5-(2,2,2-Trifluoro-ethoxy)-pyridine-2-carboxylic acid [3-((S)-2-amino-1,4-dimethyl-6-oxo-1,4,5,6-tetrahydro-pyrimidin-4-yl)-phenyl]-amide 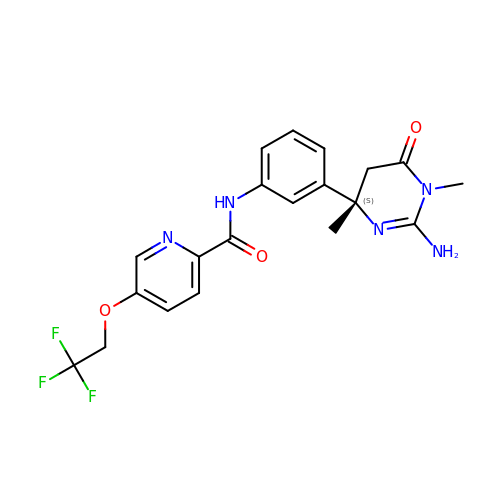| C20 H20 F3 N5 O3 | ZJFIBYCNZHIVEL-IBGZPJMESA-N3,4-difluoro-N-[(1S)-1-{1-[(2R)-4-(hydroxyamino)-4-oxo-1-(5,6,7,8-tetrahydronaphthalen-2-yl)butan-2-yl]-1H-1,2,3-triazol-4-yl}ethyl]benzamide | C25 H27 F2 N5 O3 | 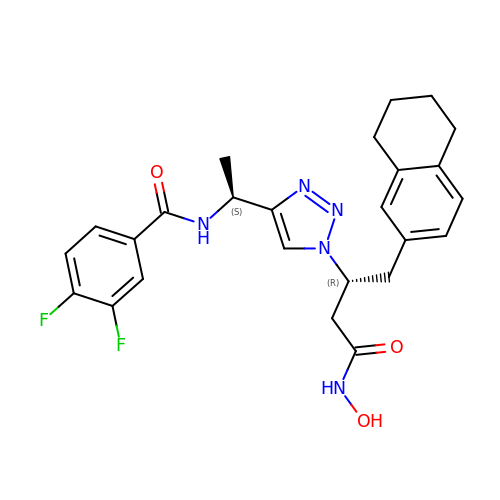VQGQRXDQPMXXSZ-MGPUTAFESA-N> APVRSLNCTLRDSQQKSLVMSGPYELKALHLQGQDMEQQVVWSMSFVQGEESNDKIPVALGLKEKNLYLSCVLKDDKPTLQLESVDPKNYPKKKMEKR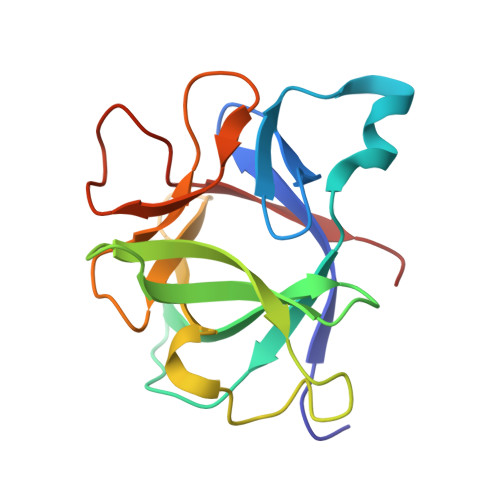FVFNKIEINNKLEFESAQFPNWYISTSQAENMPVFLGGTKGGQDITDFTMQFVSS3-amino-N-(3-fluorophenyl)-6-thiophen-2-ylthieno[2,3-b]pyridine-2-carboxamide | 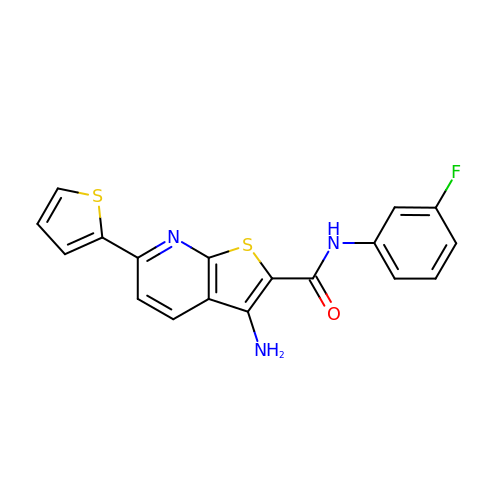C18 H12 F N3 O S2 | UCTSEHMMSSIODN-UHFFFAOYSA-N>[8x]MKVGINGFGRIGRQVFRILHSRGVEVALINDLTDNKTLAHLLKYDSIYHRFPGEVAYDDQYLYVDGKAIRATAVKDPKEIPWAEAGVGVVIESTGVFTDADKAKAHLEGGAKKVIITAPAKGEDITIVMGVNHEAYDPSRHHIISNASCTTNSLAPVMKVLEEAFGVEKALMTTVHSYTNDQRLLDLPHKDLRRARAAAINIIPTTTGAAKATALVLPSLKGRFDGMALRV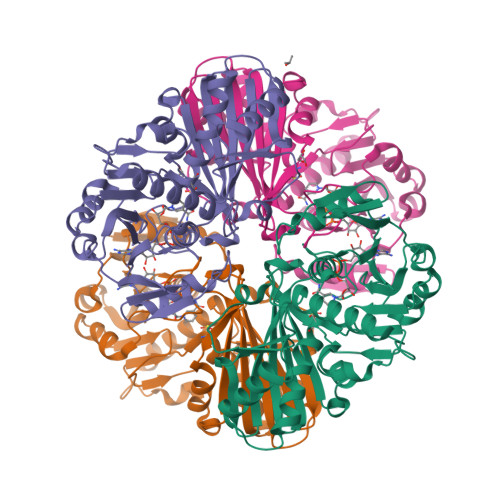PTATGSISDITALLKREVTAEEVNAALKAAAEGPLKGILAYTEDEIVLQDIVMDPHSSIVDAKLTKALGNMVKVFAWYDNEWGYANRVADLVELVLRKGV> MKILVAVKQTAALEE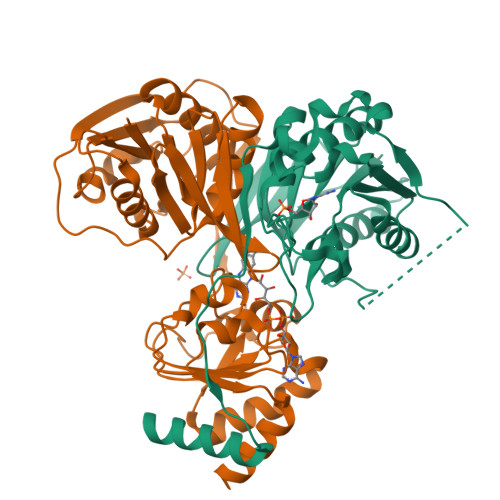DFEIREDGMDVDEDFMMYDLNEWDDFSLEEAMKIKESSDTDVEVVVVSVGPDRVDESLRKCLAKGADRAVRVWDDAAEGSDAIVVGRILTEVIKKEAPDMVFAGVQSSDQAYASTGISVASYLNWPHAAVVADLQYKPGDNKAVIRRELEGGMLQEVEINCPAVLTIQLGINKPRYASLRGIKQAATKPIEEVSLADIGLSANDVGAAQSMSRVRRMYIPEKGRATMIEGTISEQAAKIIQIINEFKGA;> MSKILVIAEHRRNDLRPVSLELIGAANGLKKSGEDKVVVAVIGSQADAFVPALSVNGVDELVVVKGSSIDFDPDVFEASVSALIAAHNPSVVLLPHSVDSLGYASSLASKTGYGFATDVYIVEYQGDELVATRGGYNQKVNVEVDFPGKSTVVLTIRPSVFKPLEGAGSPVVSNVDAPSVQSRSQNKDYVEVGGGNDIDITTVDFIMSIGRGIGEETNVEQFRELADEAGATLCCSAPIADAGWLPKSRQVGQSGKVVGSCKLYVAMGISGSIQHMAGMKHVPTIIAVNTDPGASIFTIAKYGIVADIFDIEEELKAQLAA E. coli clinical isolates express the FimH adhesin, which consists of a mannose-specific lectin domain connected via a pilin domain to the tip of type 1 pili. The FimH lectin binds specifically to mannose moieties displayed on glycoproteins at the luminal surface of epithelial cells. Mannose binds in a deep and polar pocket at the N-terminal end of FimH, in which the amino acids Phe1, Asn46, Asp47, Asp54, Gln133, Asn135, Asp140 and Phe142 create a dense network of 12 hydrogen bonds with each hydroxyl group of the pyran­ose ring except that at the α-anomeric position of mannose. The interaction of the aglycones with the tyrosine gate formed by two tyrosines (Tyr48 and Tyr137) at the entrance to the FimH binding site contributes significantly to their affinity, for example with a 400-fold increase for HM compared with α-d-manno­pyranoside.

To establish a detailed interaction profile of the tyrosine-gate residues and to rationalize the binding affinities of various FimH antagonists, we generated single-residue FimH mutants in which one of the two tyrosine-gate residues was mutated to alanine (Y48A and Y137A). In the Y48A FimH crystal structure, a large increase in the dynamics of the alkyl chain of heptyl α-d-O-mannopyranoside attempts to compensate for the absence of the aromatic ring; however, the highly energetic and stringent mannose-binding pocket of wild-type FimH is largely maintained. The affinity for AM is only slightly reduced in the mutants compared with the WT, although a decrease in the enthalpic contribution in Y48A is indicative of a loss of interactions. To summarize, the Y137A mutant samples a wider range of dihedral angles with lower energy than WT FimH, whereas at position 48 the sampling range of dihedral angles is restricted upon mutation to alanine. The energy level of the Y48A mutant is less impacted compared with the WT, congruent with the low impact of this mutation on the affinity of FimH towards BF and HM. In the Y48A mutant, the backbone dihedral angle distributions of residues 47 and 48, but not of Pro49, undergo a change. The Y48A mutation has some, but a smaller, effect on the different studied parameters and the ensemble adjusts more easily to these changes, in accordance with the enthalpy–entropy compensation seen in ITC measurements.

>FACKTANGTAIPIGGGSANVYVNLAPVVNVGQNLVVDLSTQIFCHNDAPETITDYVTLQRGSAYGGVLSNFSGTVKYSGSSYPFPTTSETPRVVYNSRTDKPWPVALYLTPVSSAGGVAIKAGSLIAVLILRQTNNYNSDDFQFVWNIYANNDVVVPT[2x]> NNDDPVENFVESTLKEVLVVPDTKPSGPQHTTKPSILGAMEIGASSNATPESTIETR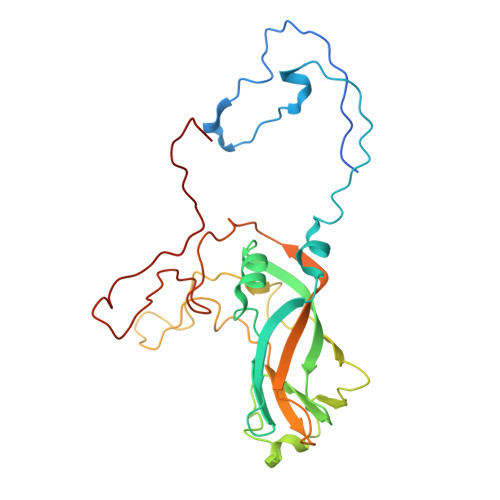YVYNTNTNAEADVEMFLGRSALWGKVTLTRQYAKWEINFQEQAHIRKKFEFFTYLRFDMEVTIVTNNKGLMQIMFVPPGIDHPETHDDRKWDSASNPSVFFQPKSGFPRFTIPFTGLASAYYMFYDGYDKPKGSDNNEYGIAPTNDMGLLCFRTLDNSGGNDVKIYVKPKHITAWVPRPPRATQYTHKYSTNYHYKPNSSGPDEHVLKDRHFIKTRPLISSA> ITLKYNYTVT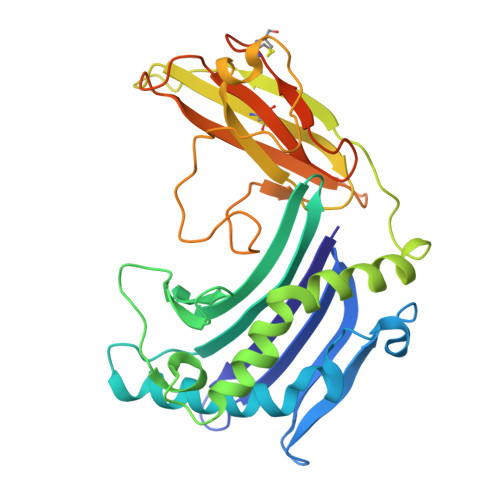LKDDGLYDGVFYDHYNDQLVTKISYNHETRHGNVNFRADWFNISRSPHTPGNDYNFNFWYSLMKETLEEINKNDSTKTTSLSLITGCYETGLLFGSYGYVETANGPLARYHTGDKRFTKMTHKGFPKVGMLTVKNTLWKDVKAYLGGFEYMGCSLAILDYQKMAKGKIPKDTTPTVKVTGNELEDGNMTLECTVNSFYPPDVITKWIESEHFKGEYKYVNGRYYPEWGRKSNYEPGEPGFPWNIKKDKDANTYSLTDLVRTTSKMSSQPVCVVFHDTLEAQVYTCSEGCNGELYDHLYRKTEEGEGGSHHHHHH2-methoxy-4-(prop-2-en-1-yl)phenol | 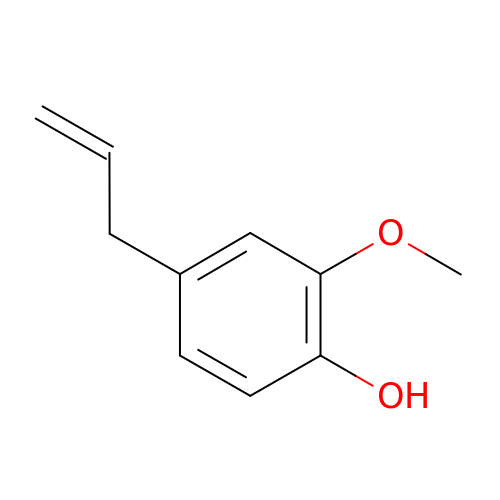C10 H12 O2 | RRAFCDWBNXTKKO-UHFFFAOYSA-N PLD3 is synthesized as a type II transmembrane protein and proteolytically cleaved in lysosomes, yielding a soluble active form. The deficiency of PLD3 leads to the slowed degradation of nucleic acids in lysosomes and chronic activation of nucleic acid-specific intracellular toll-like receptors. PLD3 has a typical phospholipase fold and forms homodimers with two independent catalytic centers via a newly identified dimerization interface. While crystal structures for RNaseT2 and DNase II are available and provide important insight into the molecular details and function of both enzymes, no experimentally determined structural information is available for the 5′ exonucleases PLD3 or PLD4. Both PLD3 and PLD4 belong to the phospholipase-D (PLD) family of phosphodiesterases, a protein family that shares a common biochemical mechanism and an H(X)K(X4)D (HKD) signature motif within their active site.

To gain insight into hPLD3 architecture, we determined the crystal structure of hPLD3 in the substrate-free (apo) form to a resolution of 1.5 Å. The asymmetric unit contained two PLD3 molecules. In both molecules, amino acids 72–98 and 101–490 were well explained in the electron density, whereas residues 61–71 and 99–100 were not visible, likely due to their exposure to the solvent providing them with higher flexibility. The two hPLD3 molecules in the asymmetric unit formed a homodimer via helices α10 and α11, with an interface area of 1042 Å2. The hPLD3 apo structure harbors a bound phosphate in the active site, which is coordinated by five direct hydrogen bonds with the HKD/HKE motif residues His201, Lys203, Asn218, His416, and water-mediated contacts of Lys418 and Asn432. In line with the mass spectrometry data, a high mannose-type sugar (Man5GlcNAc2) was well visible in the electron density at Asn284. The electron density also indicated that the side chain of Cys300 was oxidized to sulfonic acid. The cysteine sulfonic acid (OCS) residue is located in a deep pocket 20 Å away from the active site and is coordinated by the side chain of Ser294, the carbonyl oxygen of Pro296 and water molecules. In the same deep cavity of OCS300, we found electron density for a large cation that was coordinated to the oxidized cysteine side chain via a water molecule. Careful evaluation of the electron density in combination with an X-ray fluorescence scan of the crystal used for data collection of the hPLD3 apo structure indicated that this density corresponds to a manganese ion.

>[2x]QRPAPCYDPCEAVLVESIPEGLDFPNASTGNPSTSQAWLGLLAGAHSSLDIASFYWTLTNNDTHTQEPSAQQGEEVLRQLQTLAPKGVNVRIAVSKPSGPQPQADLQALLQSGAQVRMVDMQKLTHGVLHTKFWVVDQTHFYLGSANMDWRSLTQVKELGVVMYNCSCLARDLTKIFEAYWFLGQAGSSIPSTWPRFYDTRYNQETPMEICLNGTPALAYLASAPPPLCPSGRTPDLKALLNVVDNARSFIYVAVMNYLPTLEFSHPHRFWPAIDDGLRRATYERGVKVRLLISCWGHSEPSMRAFLLSLAALRDNHTHSDIQVKLFVVPADEAQARIPYARVNHNKYMVTERATYIGTSNWSGNYFTETAGTSLLVTQNGRGGLRSQLEAIFLRDWDSPYSHDLDTSADSVGNACRLLAAQ>GASPPSPPRGIKVSEVTTRTARLSWQSPYGNGDNTVVTYIVRY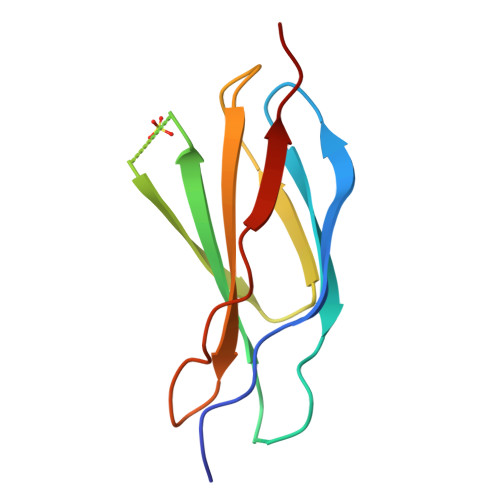WRDEESRSQLHQLTFQVTSANLKDLHPGTSYAVQILAENDVGASIPSRLVQFRTIEE[2x]>MLESKLKAPVFTATTQGDHYGEFVLEPLERGFGVTLGNPLRRILLSSIPGTAVTSVYIEDVLHEFSTIPGVKEDVVEIILNLKELVVRFLDPRWRTTLILRAEGPKEVRAVDFTPSADVEIMNPDLHIATLEEGGKLYMEVRVDRGVGYVPAERHGIKDRINAIPVDAIFSPVRRVAFQVEDTRLGQRTDLDKLTLRIWTDGSVTPLEALNQAVAILKEHLNYFANPEASLLPTPEVSKGEKRESAEEDLDLPLEELGLSTRVLHSLKEEGIESVRALLALNLKDLRNIPGIGERSLEEIRQALAKKGFTLKE[2x];> MKIKRFGRIREVIPLPPLTEIQVESYKKALQADVPPEKRENVGIQAAFKETFPIEEGDKGKGGLVLDFLEYRIGDPPFSQDECREKDLTYQAPLYARLQLIHKDTGLIKEDEVFLGHLPLMTEDGSFIINGADRVIVSQIHRSPGVYFTPDPARPGRYIASIIPLPKRGPWIDLEVEASGVVTMKVNKRKFPLVLLLRVLGYDQETLVRELSAYGDLVQGLLDEAVLAMRPEEAMVRLFTLLRPGDPPKKDKALAYLFGLLADPKRYDLGEAGRYKAEEKLGVGLSGRTLVRFEDGEFKDEVFLPTLRYLFALTAGVPGHEVDDIDHLGNRRIRTVGELMADQFRVGLARLARGVRERMVMGSPDTLTPAKLVNSRPLEAALREFFSRSQLSQFKDETNPLSSLRHKRRISALGPGGLTRERAGFDVRDVHRTHYGRICPVETPEGANIGLITSLAAYARVDALGFIRTPYRRVKNGVVTEEVVYMTASEEDRYTIAQANTPLEGDRIATDRVVARRRGEPVIVAPEEVEFMDVSPKQVFSLNTNLIPFLEHDDANRALMGSNMQTQAVPLIRAQAPVVMTGLEERVVRDSLAALYAEEDGEVVKVDGTRIAVRYEDGRLVEHPLRRYARSNQGTAFDQRPRVRVGQRVKKGDLLADGPASEEGFLALGQNVLVAIMPFDGYNFEDAIVISEELLKRDFYTSIHIERY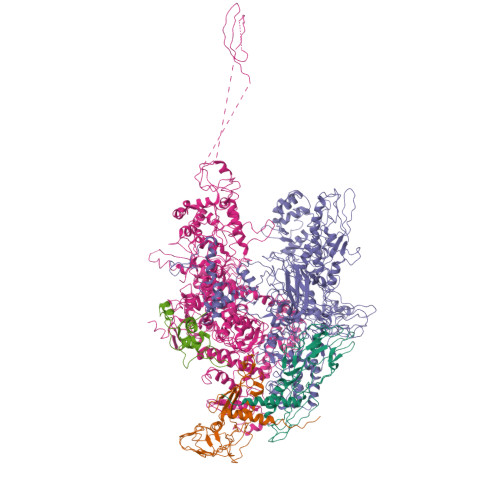EIEARDTKLGPERITRDIPHLSEAALRDLDEEGIVRIGAEVKPGDILVGRTSFKGEQEPSPEERLLRSIFGEKARDVKDTSLRVPPGEGGIVVGRLRLRRGDPGVELKPGVREVVRVFVAQKRKLQVGDKLANRHGNKGVVAKILPVEDMPHLPDGTPVDVILNPLGVPSRMNLGQILETHLGLAGYFLGQRYISPVFDGATEPEIKELLAEAFNLYFGKRQGEGFGVDKREKEVLARAEKLGLVSPGKSPEEQLKELFDLGKVVLYDGRTGEPFEGPIVVGQMFIMKLYHMVEDKMHARSTGPYSLITQQPLGGKAQFGGQRFGEMEVWALEAYGAAHTLQEMLTIKSDDIEGRNAAYQAIIKGEDVPEPSVPESFRVLVKELQALALDVQTLDEKDNPVDIFEGLASKR;> MKKEVRKVRIALASPEKIRSWSYGEVEKPETINYRTLKPERDGLFDERIFGPIKDYECACGKYKRQRFEGKVCERCGVEVTRSIVRRYRMGHIELATPAAHIWFVKDVPSKIGTLLDLFATELEQVLYFNKYIVLDPKGAVLDGVPVEKRQLLTDXXXXXXXXXXXXXXXXXXXXXXXXXXXXXXXXXXXXIDARMGAEAIQELLKELDLEKLERELLEEMKHPSRARRAKARKRLEVVRAFLDSGNRPEWMILEAVPVLPPDLRPMVQVDGGRFATSDLNDLYRRLINRNNRLKKLLAQGAPEIIIRNEKRMLQEAVDAVIDNGRRGSPVTNPGSERPLRSLTDILSGKQGRFRQNLLGKRVDYSGRSVIVVGPQLKLHQCGLPKRMALELFKPFLLKKMEEKAFAPNVKAARRMLERQRDIKDEVWDALEEVIHGKVVLLNRAPTLHRLGIQAFQPVLVEGQSIQLHPLVCEAFNADFDGDQMAVHVPLSSFAQAEARIQMLSAHNLLSPASGEPLAKPSRDIILGLYYITQVRKEKKGAGMAFATPEEALAAYERGEVALNAPIVVAGRETSVGRLKFVFANPDEALLAVAHGLLDLQDTVTTRYLGRRLETNPGRILFARIVGEAVGDEKVAQELIQMDVPQEKNSLKDLVYQAFLRLGMEKTARLLDALKYYGFTLSTTSGIITIGIDDAVIPEEKQRYLEEADRKLRQIEQAYEMGFLTDRERYDQVIQLWTETTEKVTQAVFNNFEENYPFNPLYVMAQSGARGNPQQIRQLCGMRGLMQKPSGETFEVPVRSSFREGLTVLEYFISSHGARKGGADTALRTADSGYLTRKLVDVAHEIVVREADCGTTKYISVPLFQMDEVTRTLRLRKRSDIESGLYGRVLAREVEALGRRLEEGRYLSLEDVHFLIKAAEAGEVREVPVRSPLTCQTRYGVCQKCYGYDLSMARPVSIGEAVGVVAAESIGEPGTQLTMRTFHTGGVAVGTDITQGLPRVIELFEARRPKAKAVISEIDGVVRIEEGEDRLSVFVESEGFSKEYKLPKDARLLVKDGDYVEAGQPLTRGAIDPHQLLEAKGPEAVERYLVDEIQKVYRAQGVKLHDKHIEIVVRQMLKYVEVTDPGDSPLLEGQVLEKWDVEALNERLIAEGKVPVAWKPLLMGVTKSALSTKSWLSAASFQNTTHVLTEAAIAGKKDELIGLKENVILGRLIPAGTGSDFVRFTQVVDQRTLKAIEEARKEAVEAKEKEAPRRPVRREQPGKGL;> MAEPGIDKLFGMVDSKYRLTVVVAKRAQQLLRHRFKNTVLEPEERPKMRTLEGLYDDPNAVTWAMKELLTGRLFFGENLVPEDRLQKEMERLYPTEEEA TERT-BUTYL D-ALPHA-GLUTAMINATE | C9 H18 N2 O3 | 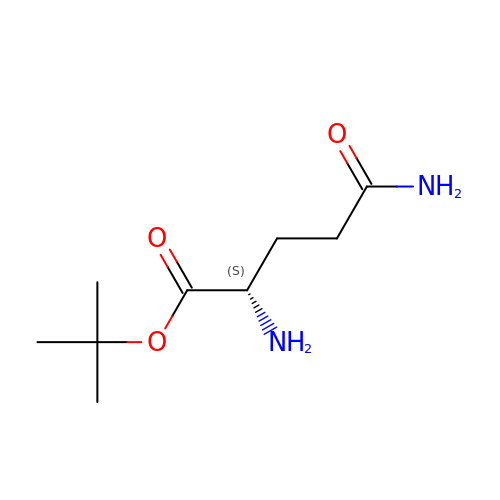VVOPSEUXHSUTJS-LURJTMIESA-N5-(4-methoxybutyl)-N-(2-methylpropyl)-N-[(3S,5R)-5-(morpholine-4-carbonyl)piperidin-3-yl]-1-phenyl-1H-1,2,3-triazole-4-carboxamide | C28 H42 N6 O4 | 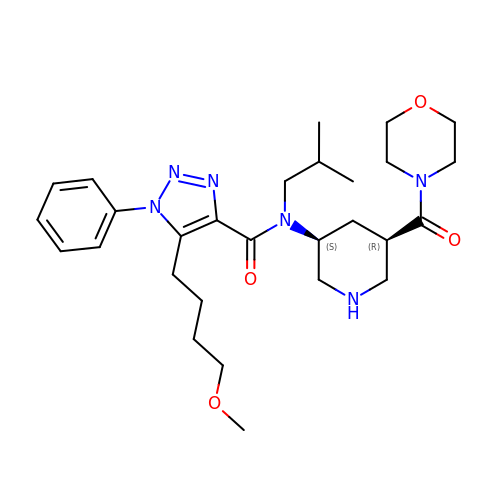SEGBKNMSWABOBA-VWNXMTODSA-N>[4x]GPLGSGFTVLSTKSLFLGQKLQVVQADIASIDSDAVVHPTNTDFYIGGEVGSTLEKKGGKEFVEAVLELRKKNGPLE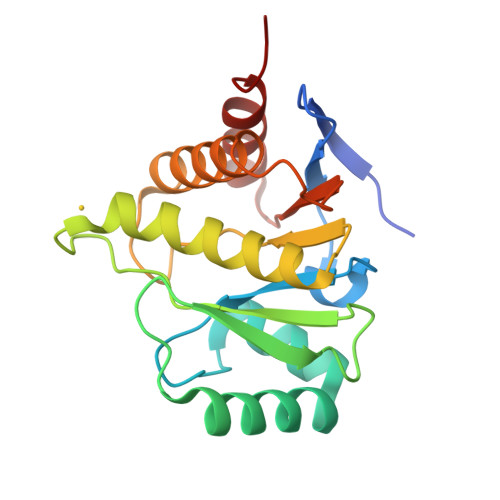VAGAAVSAGHGLPAKFVIHCNSPVWGSDKCEELLEKTVKNCLALADDRKLKSIAFPSIGSGRNGFPKQTAAQLILKAISSYFVSTMSSSIKTVYFVLFDSESIGIYVQEMAKLDAN>[4x]GRNRRRTVRSEGIDPEKAKLYQAPYFEKSEDEMNLITKLLTHNVLFSFLNTK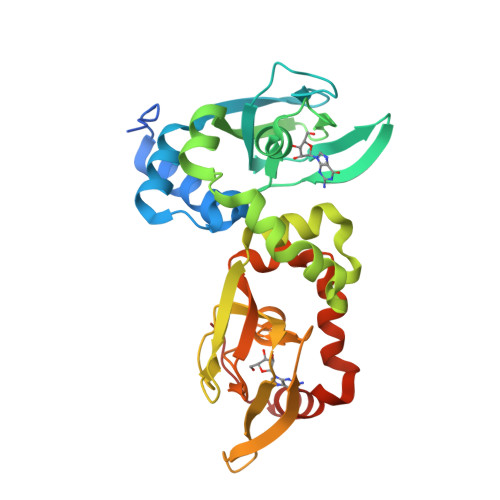DIKVVAGAMQRATFKHDDCIMEAGQTTCNKLYIIQSGHADIIKEGQKVYLKTEGTAVGELELMYDTPVVATVKVCTDELIAWVLDRDTYRNLVMGTAIRRRETYIQFLANVPFLGGLDSYEKLQLADALSSEEFSPGEYIIHYGEEGEWLYIIMEGTVEVIGRDADGEPTKVCEFTQGDHIGELEFLNNHRTVADVVATTHVITAKLNRRHFEMCLGPVIDVLKRCADDPKYEYYQNVLKTGAAQPSYVDDV> MHSQMLKGVLEGCILYIISQEEVYGYELSTKLNKHGFTFVSEGSIYPLLLRMQKEKLIEGTLKASSLGPKRKYYHITDKGLEQLEEFKQSWGMVSTTVNNLLQGESRWS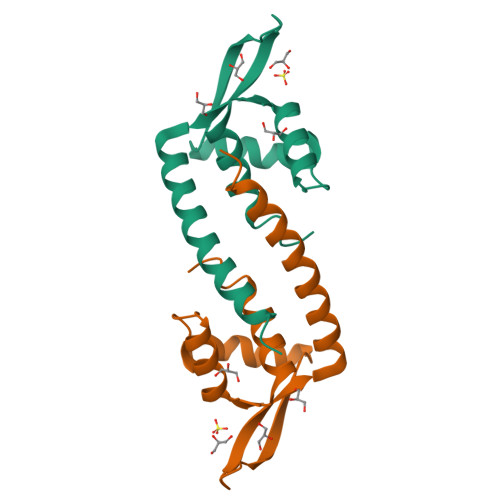HPQFEK> MWPKRLTKAHWFEIQHIQPSPLQCNRAMSGINNYTQHCKHQNTFLHDSFQNVAAVCDLLSIVCKNRRHNCHQSSKPVNMTDCRLTSGKYPQCRYSAAAQYKFFIVACDPP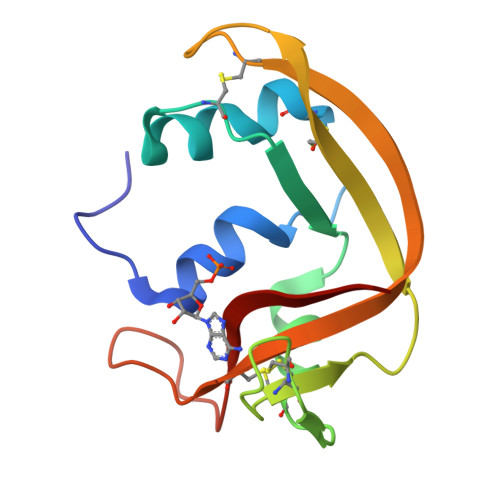QKSDPPYKLVPVHLDSIL>[2x]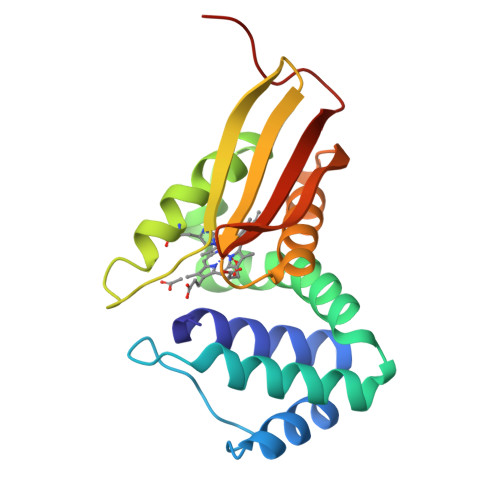MKGTIVGTWIKTLRDLYGNDVVDESLKSVGWEPDRVITPLEDIDDDEVRRIFAKVSEKTGKNVNEIWREVGRQNIKTFSEWFPSYFAGRRLVNFLMMMDEVHLQLTKMIKGATPPRLIAKPVAKDAIEMEYVSKRKMYDYFLGLIEGSSKFFKEEISVEEVERGEKDGFSRLKVRIKFKNPVFEYKKN> MSPEEWTYLVVLLISIPIGFLFKKAGPGLKRWGAAAVGLGLTLFTCGPHTLHSLVTILGTWALIQAQPCSCHALALAWTFSYLLFFRALSLLGLPTPTPFTNAVQ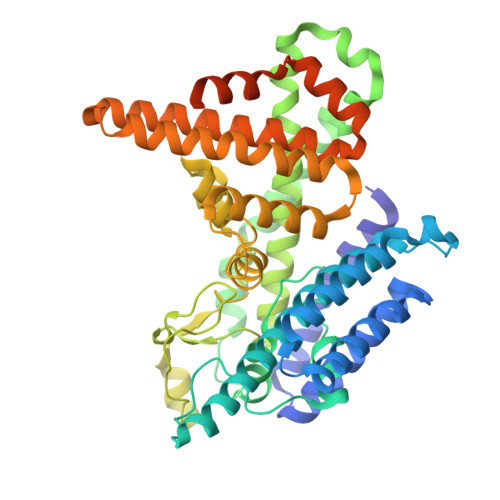LLLTLKLVSLASEVQDLHLAQRKEMASGFSKGPTLGLLPDVPSLMETLSYSYCYVGIMTGPFFRYRTYLDWLEQPFPGAVPSLRPLLRRAWPAPLFGLLFLLSSHLFPLEAVREDAFYARPLPARLFYMIPVFFAFRMRFYVAWIAAECGCIAAGFGAYPVAAKARAGGGPTLQCPPPSSPEKAASLEYDYETIRNIDCYSTDFCVRVRDGMRYWNMTVQWWLAQYIYKSAPARSYVLRSAWTMLLSAYWHGLHPGYYLSFLTIPLCLAAEGRLESALRGRLSPGGQKAWDWVHWFLKMRAYDYMCMGFVLLSLADTLRYWASIYFCIHFLALAALGLGLALGGGSPSRRKAASQPTSLAPEKLREELEACGIENLYFQ> NTKYNKEFLLYLAGFVDGDGSIIAQIKPNQSGKFKHKLSL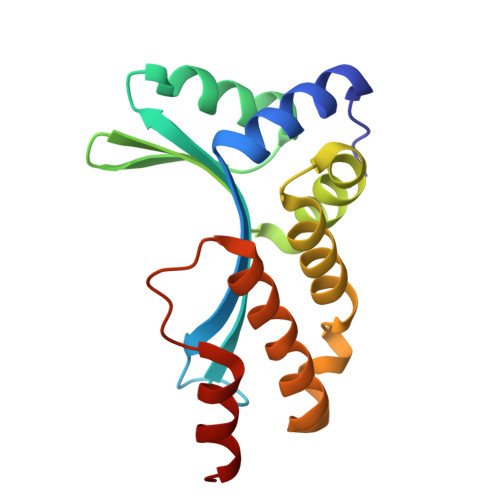TFKVTQKTQRRWFLDKLVDEIGVGYVYDSGSVSNYYLSEIKPLHNFLTQLQPFLKLKQKQANLVLKIIEQLPSAKESPDKFLEVCTWVDQVAALNDSKTRKTTSETVRAVLDSL>[4x]MKEFYLTVEQIGDSIFERYIDSNGRERTREVEYKPSLFAHCPESQATKYFDIYGKPCTRKLFANMRDASQWIKRMEDIGLEALGMDDFKLAYLSDTYNYEIKYDHTKIRVANFDIEVTSPDGFPEPSQAKHPIDAITHYDSIDDRFYVFDLLNSPYGNVEEWSIEIAAKLQEQGGDEVPSEIIDKIIYMPFDNEKELLMEYLNFWQQKTPVILTGWNVESFAIPYVYNRIKNIFGESTAKRLSPHRKTRVKVIENMYGSREII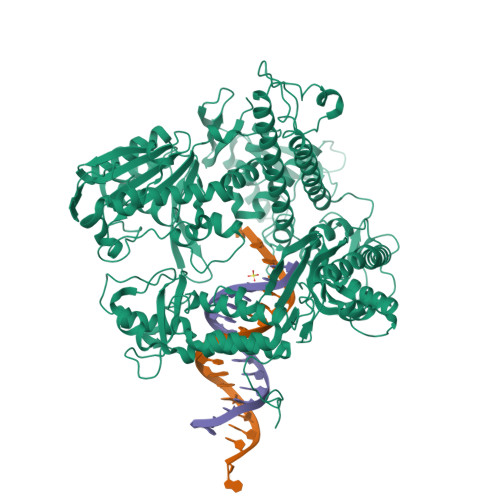TLFGISVLDYIDLYKKFSFTNQPSYSLDYISEFELNVGKLKYDGPISKLRESNHQRYISYNIIAVYRVLQIDAKRQFINLSLDMGYYAKIQIQSVFSPIKTWDAIIFNSLKEQNKVIPQGRSHPVQPYPGAFVKEPIPNRYKYVMSFDLTSLYPSIIRQVNISPETIAGTFKVAPLHDYINAVAERPSDVYSCSPNGMMYYKDRDGVVPTEITKVFNQRKEHKGYMLAAQRNGEIIKEALHNPNLSVDEPLDVDYRFDFSDEIKEKIKKLSAKSLNEMLFRAQRTEVAGMTAQINRKLLINSLYGALGNVWFRYYDLRNATAITTFGQMALQWIERKVNEYLNEVCGTEGEAFVLYGDTDSIYVSADKIIDKVGESKFRDTNHWVDFLDKFARERMEPAIDRGFREMCEYMNNKQHLMFMDREAIAGPPLGSKGIGGFWTGKKRYALNVWDMEGTRYAEPKLKIMGLETQKSSTPKAVQKALKECIRRMLQEGEESLQEYFKEFEKEFRQLNYISIASVSSANNIAKYDVGGFPGPKCPFHIRGILTYNRAIKGNIDAPQVVEGEKVYVLPLREGNPFGDKCIAWPSGTEITDLIKDDVLHWMDYTVLLEKTFIKPLEGFTSAAKLDYEKKASLFDMFDFHHH>MSLALTHDKNGDAHYDVISAFQKSIRGSDVDAALHYLARLVEAGDLASICRRLMVIGYEDIGLGNPAAAARTVNAVLAAEKLGLPEARIPLADVVVDLCL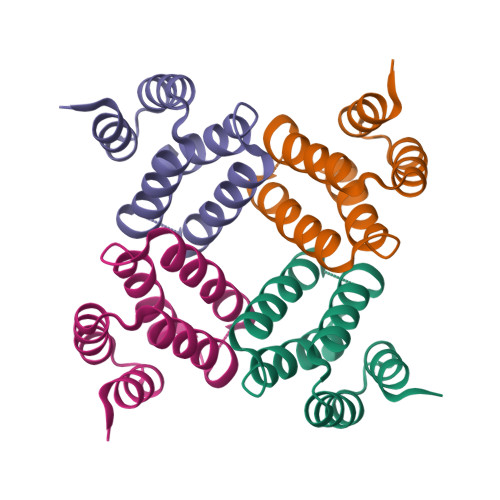SPKSEGHHHHHH[4x]> IFPKQYPIINFTTAGATVQSYTNFIRAVRGRLTTGADVRHEIPVLPNRVGLPINQRFILVELSNHAELSVTLALDVTNAYVVGYRAGNSAYFFHPDNQEDAEAITHLFTDVQNRYTFAFGGNYDRLEQLAGNLRENIELGNGPLEEAISALYYYSTGGTQLPTLARSFIICIQMISEAARFQYIEGEMRTRIRYNRRSAPDPSVITLENSWGRLSTAIQESNQGAFASPIQLQRRNGSKFSVYDVSILIPIIALMVYRCAPPPSS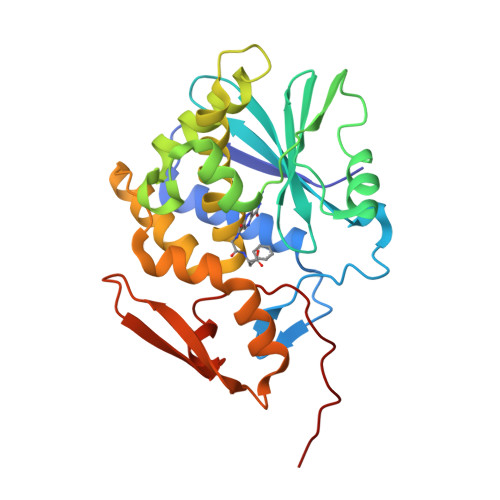QF>[11x]MAPYSVVASVLAAAPPQQSGSVRQLPSTINRAITQRSQSRHVASASSASSPTTMLEERDN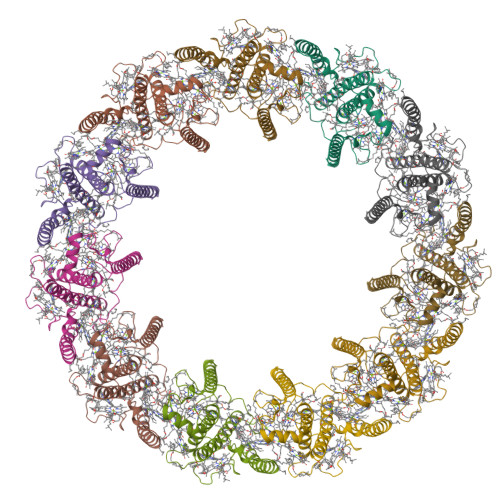LWEIGGPYWWPFSSFTPPAHLDGSLPGDRGFDPFSLGTSWGQPPVDVSDPNYDESRLRWLLEGELYNGRLAMLAVVGVLTVEAQGKGPWWEIPGNLNLFGTPYVVAVVGGHLAFALLEKKRLENFRETGEAGHFGAARFDPLDLTEANPLGTDYNRQAEVRNCRLAMLTFLGFSVQAWVTGKGPIENAKDHLASPFEANIFTYGDRGTNVVAIFSAFAAVMHIAELAREKKAEDKPRSRNRTLSGSS>[2x]MGSLVNRKQLEKMANVRFRTQEDEYVAILDALEEYHNMSENTVVEKYLKLKDINSLTDIYIDTYKKSGRNKALKKFKEYLVTEVLELKNNNLTPVEKNLHFVWIGGQINDTAINYINQWKDVNSDYNVNVFYDSNAFLINTLKKTVVESAINDTLESFRENLNDPRFDYNKFFRKRMEIIYDKQKNFINYYKAQREENPELIIDDIVKTYLSNEYSKEIDELNTYIEESLNKITQNSGNDVRNFEEFKNGESFNLYEQELVERWNLAAASDILRISALKEIGGMYLDVDMLPGIQPDLFESIEKPSSVTVDFWEMTKLEAIMKYKEYIPEYTSEHFDMLDEEVQSSFESVLASKSDKSEIFSSLGDMEASPLEVKIAFNSKGIINQGLISVKDSYCSNLIVKQIENRYKILNNSLNPAISEDNDFNTTTNTFIDSIMAEANADNGRFMMELGKYLRVGFFPDVKTTINLSGPEAYAAAYQDLLMFKEGSMNIHLIEADLRNFEISKTNISQSTEQEMASLWSFDDARAKAQFEEYKRNYFEGSLLEHHHHHH

TcdA and TcdB bacterial toxins are primary determinants of disease pathogenesis and are attractive therapeutic targets. TcdA and TcdB contain domains that use UDP-glucose to glucosylate and inactivate host Rho GTPases, resulting in cytoskeletal changes causing cell rounding and loss of intestinal integrity. The GTD domains of TcdA and TcdB catalyze transfer of a glucosyl residue to a nucleophilic threonine acceptor in Rho GTPases. Iminosugars, isofagomine and noeuromycin mimic the transition state and inhibit both TcdA and TcdB by forming ternary complexes with Tcd and UDP, a product of the TcdA- and TcdB-catalyzed reactions.

The geometry of UDP, isofagomine and noeuromycin bound to TcdB-GTD was established by solving the crystal structures. Electron densities for UDP, isofagomine and noeuromycin were also well resolved in the crystal structures. The binding of UDP and noeuromycin is similar to UDP and isofagomine interactions. However, the ion-pair interaction distance between the nitrogen cation of noeuromycin and the β-phosphate oxygen is slightly weaker at 2.7 Å. The C2-hydroxyl of the noeuromycin also interacts (3.0 Å) with a β-phosphate of the UDP. Despite the extra interaction of the noeuromycin C2-hydroxyl, the combination of this interaction and the weaker nitrogen cation to UDP interaction together caused reduced inhibition potency when compared to isofagomine. Here, noeuromycin was 7.6-fold less potent than isofagomine, thus the C2′′ hydroxyl group does not improve inhibitory activity. With UDP, isofagomine and noeuromycin gave KD = 0.067 ± 0.019 µM and a KD = 0.180 ± 0.070 µM respectively. Isofagomine and noeuromycin binding is enthalpically driven with ΔH = −10.3 ± 0.1 kcal/mol and ΔH = −5.2 ± 0.1 kcal/mol, respectively. Movement of the loop from residues Gln510 to Asp523 (10 Å) towards the binding pocket occurs on inhibitor binding and is highlighted with the black arrow.resiniferatoxin | C37 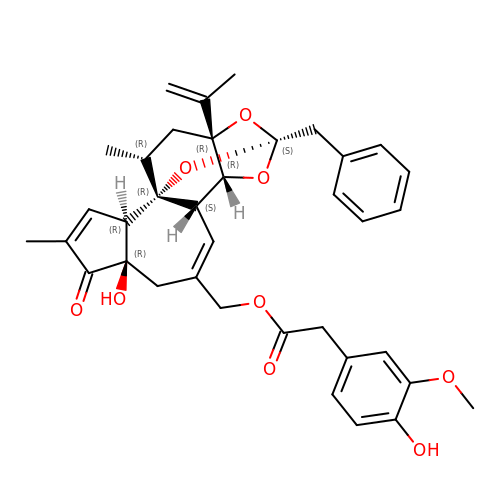H40 O9 | DSDNAKHZNJAGHN-MXTYGGKSSA-N>[8x]SENYALTTNQGVRIADDQNSLRAGS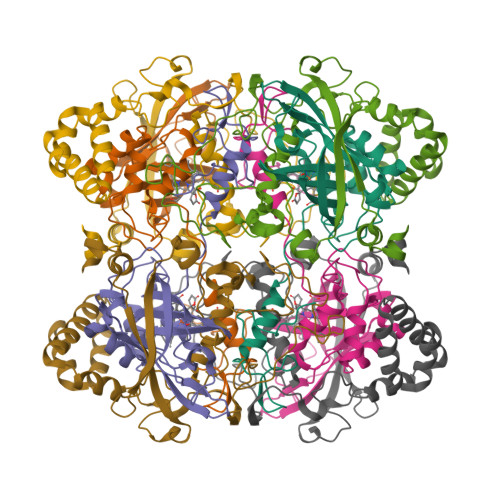RGPTLLEDFILREKITHFDHERIPERIVHARGSAAHGYFQPYKSLSDITKADFLSDPNKITPVFVRFSTVQGGAGSADTVRDIRGFATKFYTEEGIFDLVGNNTPIFFIQDAHKFPDFVHAVKPEPHWAIPQGQSAHDTFWDYVSLQPETLHNVMWAMSDRGIPRSYRTMEGFGIHTFRLINAEGKATFVRFHWKPLAGKA;>KLTGRDPDFHRRELWEAIEAGDFPEYELGFQLIPEEDEFKFDFDLLDPTKLIPEELVPVQRVGKMVLNRNPDNFFAENEQAAFHPGHIVPGLDFTNDPLLQGRLFSYTDTQISRLGGPNFHEIPINRPTCPYHNFQRDGMHRMGIDTNPANYEPNSINDNWPRETPPGPKRGGFESYQERVEGNKVRERSPSFGEYYSHPRLFWLSQTPFEQRHIVDGFSFELSKVVRPYIRERVVDQLAHIDLTLAQAVAKNLGIELT[8x]> VEGAVKTEPVDLFHPGFLNSSNYRIPALFKTKEGTLIASIDARRHGGADAPNNDIDTAVRRSEDGGKTWDEGQIIMDYPDKSSVIDTTLIQDDETGRIFLLVTHFPSKYGFWNAGLGSGFKNIDGKEYLCLYDSSGKEFTVRENVVYDKDSNKTEYTTNALGDLFKNGTKIDNINSSTAPLKAKGTSYINLVYSDDDGKTWSEPQNINFQVKKDWMKFLGIAPGRGIQIKNGEHKGRIVVPVYYTNEKGKQSSA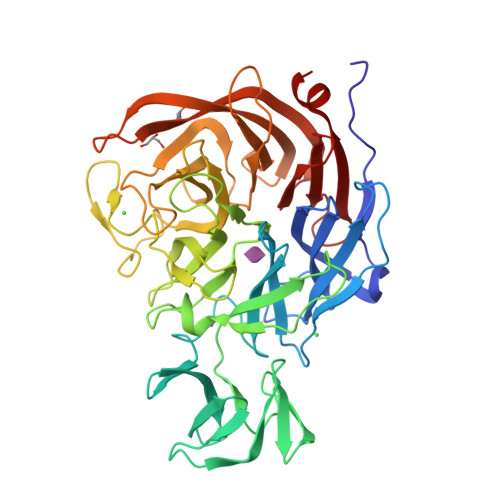VIYSDDSGKNWTIGESPNDNRKLENGKIINSKTLSDDAPQLTECQVVEMPNGQLKLFMRNLSGYLNIATSFDGGATWDETVEKDTNVLEPYCQLSVINYSQKVDGKDAVIFSNPNARSRSNGTVRIGLINQVGTYENGEPKYEFDWKYNKLVKPGYYAYSCLTELSNGNIGLLYEGTPSEEMSYIEMNLKYLESG> AFKRHIDRLPIIPADAKKHNVTCHFCIVGCGYHAYTWPINKQGGTDPQNNIFGVDLSEQQQAESDAWYSPSMYNVVKQDGRDVHVVIKPDHECVVNSGLGSVRGARMAETSFSEARNTQQQRLTDPLVWRYGQMQPTSWDDALDLVARVTAKIVKEKGEDALIVSAFDHGGAGGGYENTWGTGKLYFEAMKVKNIRIHNRPAYNSEVHGTRDMGVGELNNCYEDAELADTIVAVGTNALETQTNYFLNHWIPNLRGESLGKKKELMPEEPHEAGRIIIVDPRRTVTVNACEQTAGADNVLHLAINSGTDLALFNALFTYIADKGWVDRDFIDKSTLREGTARPPLYPARGVSEANPGHLSSFEDAVEGCRMSIEEAAEITGLDAAQIIKAAEWIGMPKEGGKRRRVMFGYEKGLIWGNDNYRTNGALVNLALATGNIGRPGGGVVRLGGHQEGYVRPSDAHVGRPAAYVDQLLIGGQGGVHHIWGCDHYKTTLNAHEFKRVYKKRTDMVKDAMSAAPYGDREAMVNAIVDAINQGGLFAVNVDIIPTKIGEACHVILPAATSGEMNLTSMNGERRMRLTERYMDP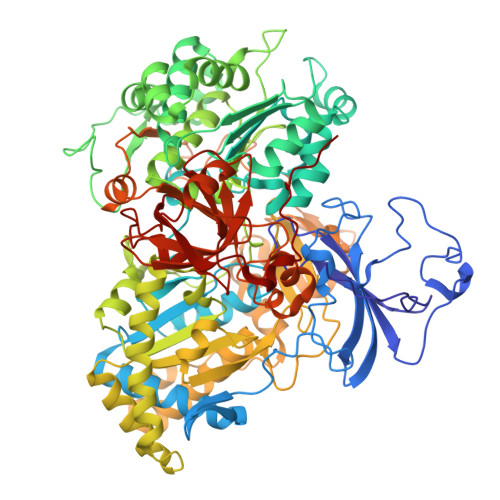PGQSMPDCLIAARLANTMERVLTEMGDVGYAAQFKGFDWQTEEDAFMDGYNKNAHGGEFVTYERLSAMGTNGFQEPATGFTDGKIEGTQRLYTDGVFSTDDGKARFMDAPWRGLQAPGKQQQKDSHKYLINNGRANVVWQSAYLDQENDFVMDRFPYPFIEMNPEDMAEAGLKEGDLVEIYNDAGATQAMAYPTPTARRGETFMLFGFPTGVQGNVTSAGTNELIIPNYKQTWGNIRKISDAPRNVAHLSFKSKEYQS(2R)-2-[(4-benzylphenoxy)methyl]pyrrolidine | C18 H21 N O 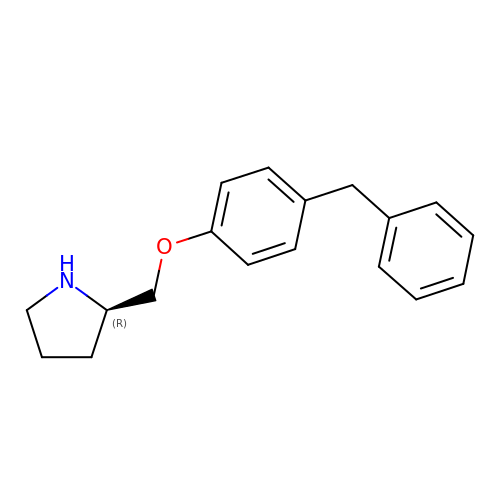| NXNMORHGFGYRDN-QGZVFWFLSA-N>MENREPPLLPARWSSAYVSYWSPMLPDDQLTSGYCWFDYERDICRIDGLFNPWSERDTGYRLWMSEVGNAASGRT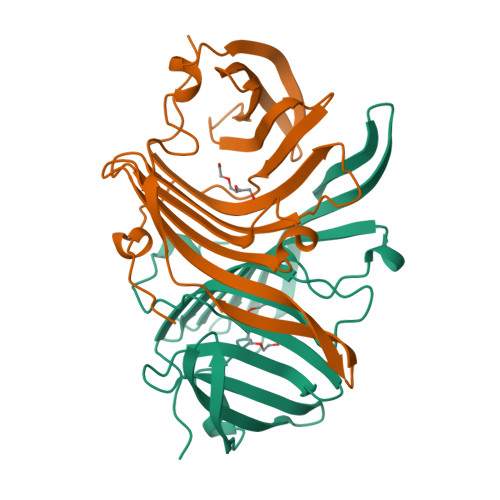WKQKVAYGRERTALGEQLCERPLDDETGPFAELFLPRDVLRRLGARHIGRRVVLGREADGWRYQRPGKGPSTLYLDAASGTPLRMVTGDEASRASLRDFPNVSEAEIPDAVFAAKRLEHHHHHH[2x]> MGITMDEEVIFETPRELISIKRIKDIPRSKDTHVFAACITSDGYPLIGARRTSFAFQAILSQQNSDSIFRVSTKLLRFMYYNELREIFRRLRKGSINNIDPHFEELILLGGKLDKKESIKDCLRRELKEESDERITVKEFGNVILKLTTRDKLFNKVYIGYCMACFINQSLEDLSHTSIYNVEIRKIKSLNDCINDDKYEYLSYI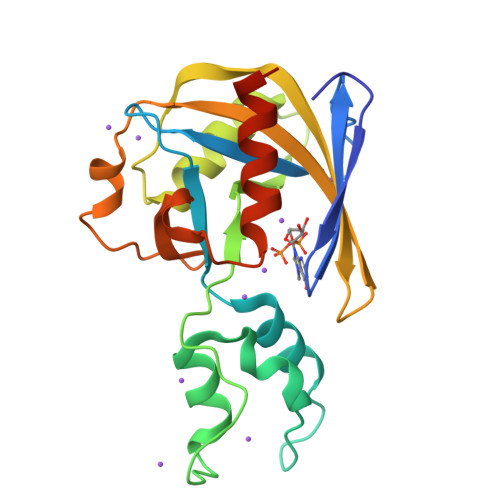YNMLVNSKLEHHHHHH Cellular retinol-binding protein 1 (CRBP1) is the primary transporter of all-trans-retinol (atROL) in the eye, and its inhibition has recently been shown to protect mouse retinas from light-induced retinal damage. We determine binding affinities for the newly identified compounds and elucidate mechanisms of their interaction with the protein by solving high-resolution X-ray structures of human CRBP1 in complex with selected inhibitors. Consistent with the fluorescence data, all of the crystallized compounds acted as competitive inhibitors of CRBP1, occupying the same binding site as atROL. Apart from specific hydrogen bonds, effective binding of retinoids or other high-affinity ligands to CRBPs requires interactions with the entry portal region of the protein, comprising α-helix I and II, as well as hairpin turns between β-strands 3–4 and 5–6.

As anticipated, the substitution of the hydrophobic 4-methylphenyl cyclopentyl group in inhibitor 1 with diphenylmethyl moieties yielded a functional CRBP1 inhibitor, denoted as compound number 5. For example, compounds that contain the 1,2,4-oxadiazole ring form a hydrogen bond between their nitrogen atom N(2) and an ordered water molecule, whose spatial position is further stabilized by the interaction with the side chain of Q128 (inhibitors 1, 3, 5, and 6). A secondary interaction site is formed between the nitrogen atom of the N-methyl group and the ordered water molecule (inhibitor 1, 5, and 6), which in turn is involved in an extended network of hydrogen bonding with the side chains of residues Y19, W106, and R104. The spatial position of these compounds reveals an overlap between the orientation of the β-ionone ring of atROL and the methylphenyl or cyclopentyl rings (inhibitors 1, 2, and 6), diphenylmethyl rings (inhibitors 3 and 5), or the tetrahydronaphthalene moiety of inhibitor 4. The stability of the main chain in the α-helices I/II and the loop between β-strands 5 and 6 correlates with the binding affinity of the tested compounds, showing a notable reduction for ligands with lower binding affinities. It is noteworthy that inhibitor 2, 3, and 5 exhibit a greater propensity to stabilize the α-helices I/II region in comparison to compounds 1, 4, and 6. Additionally, it is interesting to note that certain nonretinoid ligands have the potential to enhance conformational flexibility in segments of CRBP1 that remain well-structured even in the protein’s apo form. This phenomenon is particularly observed in inhibitors 2, 3, and 5, where their binding leads to a partial destabilization of β-strands 6 and 7. Interestingly, the magnitude of changes in conformational flexibility depends on the type of inhibitor. abn-CBD and inhibitors 2, 3, and 5 exhibited the strongest stabilizing effect on the portal region, followed by inhibitors 1, 4, and 6.

> MPVDFTGYWKMLVNENFEEYLRALDVNVALRKIANLLKPDKEIVQDGDHMIIRTLSTFRNYIMDFQVGKEFEEDLTGIDDRKCMTTVSWDGDKLQCVQKGEKEGRGWTQWIEGDELHLEMRVEGVVCKQVFKKVQHHHHHH>GHHHHHHELANNTTGFTRIIKAAGYSWKGLRAAWINEAAFRQEGVAVLLCVVIAAWLDVDAVTRVLLISSVMLVMIVELLNSAIEAVVDRIGSEYHELSGRAKDLGSAAVLIAIIDAVITWAILLWSHFG[6x]

Here, a method for presenting crystals of soluble and membrane proteins growing in the lipid cubic or sponge phase for in situ diffraction data collection at cryogenic temperatures is introduced. The method is a variant on the recently introduced in meso in situ serial crystallography (IMISX) method that enables crystallo­graphic measurements at cryogenic temperatures where crystal lifetimes are enormously enhanced whilst reducing protein consumption dramatically. The new approach has been used to generate high-resolution crystal structures of a G-protein-coupled receptor, α-helical and β-barrel transporters and an enzyme as model integral membrane proteins. Insulin and lysozyme were used as test soluble proteins.

DgkA is a kinase that resides in the inner membrane of E. coli. It is responsible for the ATP-dependent synthesis of phosphatidic acid from diacylglycerol. Crystals of this protein grow optimally in 7.8 MAG at 277 K. DgkA is therefore an example of a protein that produces crystals at a temperature other than ambient, where in situ data collection, as implemented in the IMISX method, cannot be performed conveniently at most synchrotron MX beamlines. Increasingly, we find that membrane-protein targets crystallize optimally by the in meso method at 277 K. The IMISXcryo method is ideal for such targets because the crystals can be grown at 277 K and then snap-cooled and stored in liquid nitrogen for shipping in Dewars to a synchrotron for data collection at 100 K. Complete data from the 12 crystals came from a total of 280° of data gathered at 20–40° per crystal. The highest resolution shell had a completeness of 98.6%, a CC1/2 value of 0.36 and an 〈I/σ(I)〉 of 1.00. The data-quality and refinement statistics are similar, as are the two structures, which have an r.m.s.d. value of 0.238 Å over 585 residues. These results show that the IMISXcryo method works with crystals that grow at temperatures other than ambient.N-[2-[[5-(4-fluorophenyl)-2,3-dihydroxybenzoyl]amino]ethyl]-6-hydroxypyrimidine-4-carboxamide 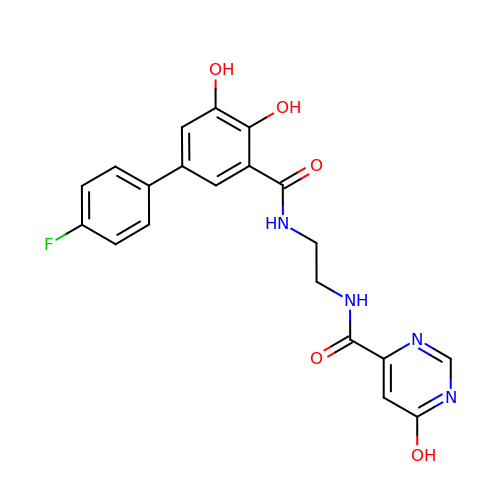| C20 H17 F N4 O5 | OVOPZHOSJPXQEE-UHFFFAOYSA-N(3-exo)-8,8-dimethyl-3-[4-(pyridin-4-yl)-1H-1,2,3-triazol-1-yl]-8-azoniabicyclo[3.2.1]octane | C16 H22 N5 | 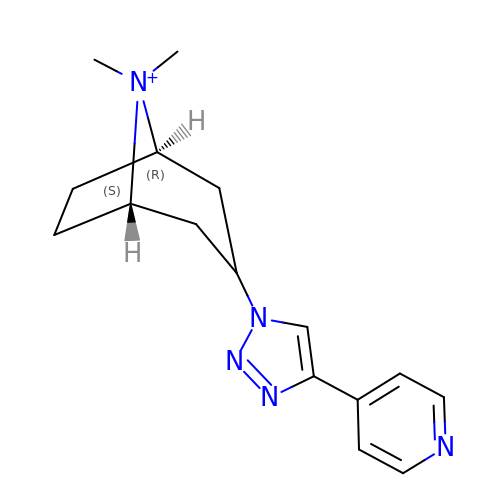IRDLJZVYUZKXLE-QKDCVEJESA-N> GSKPMEVYVSAVASPTKFWVQLIGPQSKKLDSMVQEMTSYYSSAENRAKHVLTAPYVGQIVAAVFKFDEKWYRAEIVDIMPNQYNPKEQVIDL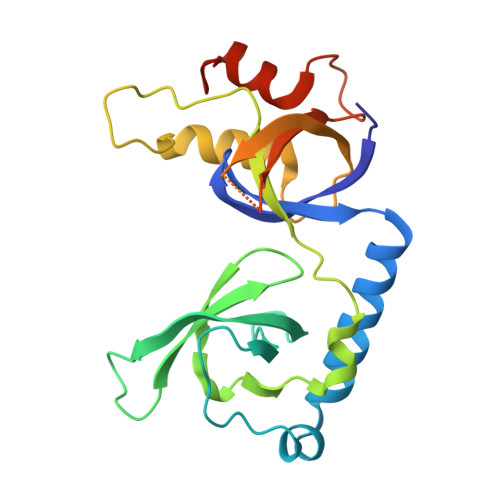YFVDYGDSEYISPADICELRTDFLTLRFQAVECFLANVKSTIQTEPITWPKSSIAKFEELTEVAHWRKLIARVVTYKERPRATTAVSAAAKEGTPLPGVELFDPADNSELNIADLMITQGFALPLDDSYP> QS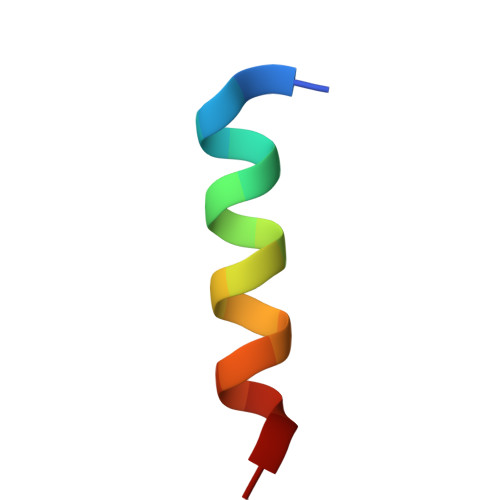INDRALSLLQRTRATK>MDHHHHHHLPNITILATGGVIAGGGDSATKSNYTVGKVGVENLVNAVPQLKDIANVKGEQVVNIGSQDMNDNVWLTLAKKINTDCDKTDGFVITHGTDTMEETAYFLDLTVKCDKPVVMVGAMRPSTSMSADGPFNLYNAVVTAADKASANRGVLVVMNDTVLDGRDVTKTNTTDVATFKSVNYGPLGYIHNGKIDYQRTPARKHTSDTPFDVSKLNELPKVGIVYNYANA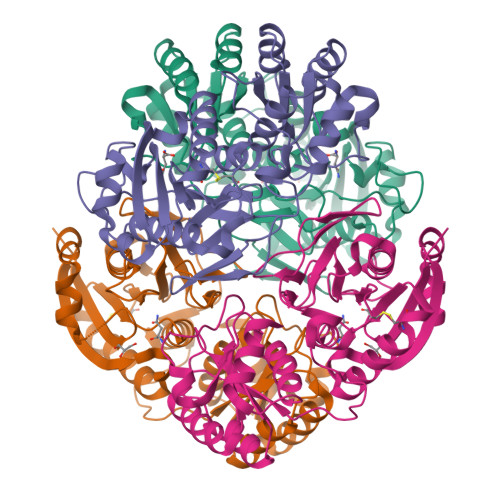SDLPAKALVDAGYDGIVSAGVGNGNLYKSVFDTLATAAKTGTAVVRSSRVPTGATTQDAEVDDAKYGFVASGTLNPQKARVLLQLALTQTKDPQQIQQIFNQY[2x]>QAQITGRPEWIWLALGTALMGLGTLYFLVKGMGVSDPDAKKFYAITTLVPAIAFTMYLSMLLGYGLTMVPFGGEQNPIYWARYADWLFTTPLLLLDLALLVDADQGTILALVGADGIMIGTGLVGALTKVYSYRFVWWAISTAAMLYILYVLFFGFTSKAESMRPEVASTFKVLRNVTVVLWSAYAVVWLIGSEGAGIVPL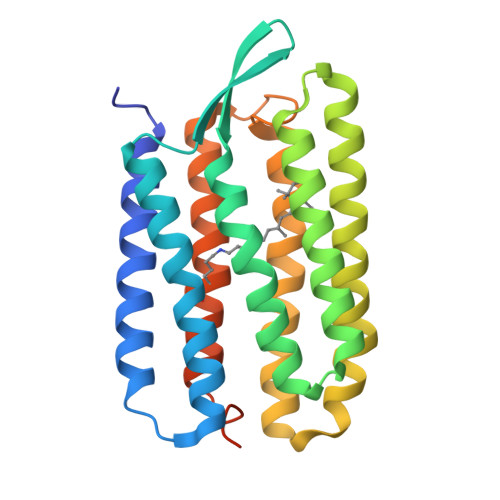NIETLLFMVLDVSAKVGFGLILLRSRAIFGEAEAPEPSAGDGAAATSD[2x]> MQASQFSAQVLDWYDKYGRKTLPWQIDKTPYKVWLSEVMLQQTQVATVIPYFERFMARFPTVTDLANAPLDEVLHLWTGLGYYARARNLHKAAQ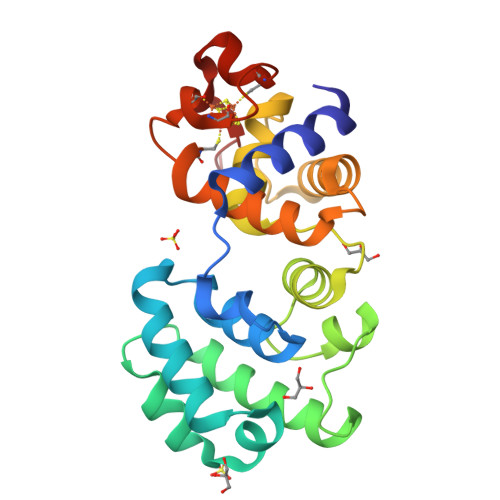QVATLHGGKFPETFEEVAALPGVGRSTAGAILSLSLGKHFPILDGNVKRVLARCYAVSGWPGKKEVENKLWSLSEQVTPAVGVERFNQAMMDLGAMICTRSKPKCSLCPLQNGCIAAANNSWALYPGKKPK> MLKMFILFLISFSWYANATDFVYRVDSRPPEEIFRDGFRSHGFNRNLQQHLRGDSC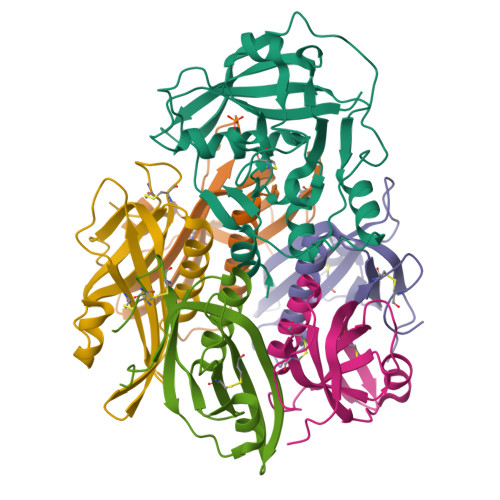AAGSRDSAFIATTTSLIETYNIARQYYSSSGFHGRLYRYRIRANNIFYPIQPSVNYLTQRGITFSGFERIMMREQNEIVAVEHIPGENIVEAVELTYDRFNSQVSDGPGTTNARYVPGSTFVNPGVIPQLVVPTVSVRERINAFGSLISACFALKGVRRDGLNKRATYYEPEFYDARGVLKEIIK;>MADYDKYFSNVQINNLSYGVYTSGGKESQFFCIGIKRDNVTLPIHNMCKVDVFGSHKQGFDAMMEMAKYYYATGESIRVYYKENVWSDSEFKKAFSTNELISLSTCSSSDYCMGPQKDTLEHHHHHH[5x]>GVALGATRVIYPAGQKQVQLAVTNNDENSTYLIQSWVENADGVKDGRFIVTPPLFAMKGKKENTLRILDATNNQLPQDRESLFWMNVKAIPSMDKSKLTENTLQLAIISRIKLYYRPAKLALPPDQAAEKLRFRRSANSLTLINPTPYYLTVTELNAGTRVLENALVPPMGESTVKLPSDAGSNITYRTINDYGALTPKMTGVME[8x];>[8x]FACKTANGTAIPIGGGSANVYVNLAPVVNVGQNLVVDLSTQIFCHNDYPETITDYVTLQRGSAYGGVLSNFSGTVKYSGSSYPFPTTSETPRVVYNSRTDKPWPVALYLTPVSSAGGVAIKAGSLIAVLILRNTNNYNSDDFQFVWNIYANNDVVVPTGGCDVSARDVTVTLPDYPGSVPIPLTVYCAKSQNLGYYLSGTTADAGNSIFTNTASFSPAQGVGVQLTRNGT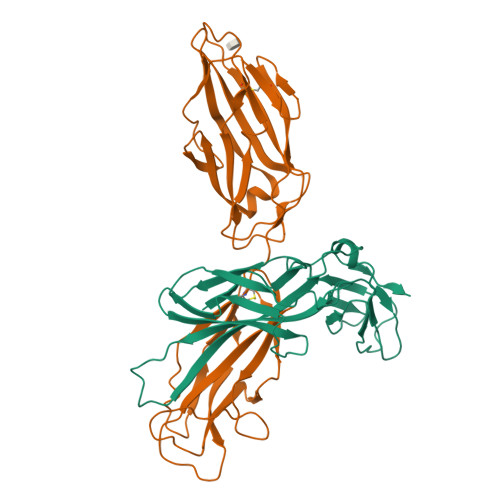IIPANNTVSLGAVGTSAVSLGLTANYARTGGQVTAGNVQSIIGVTFVYQ7-chloro-3-methyl-2H-1,2,4-benzothiadiazine 1,1-dioxide | C8 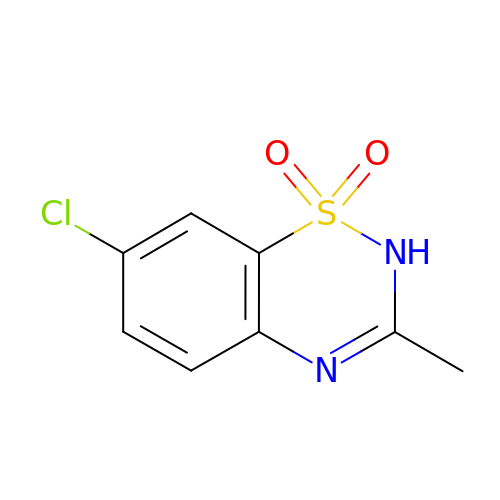H7 Cl N2 O2 S | GDLBFKVLRPITMI-UHFFFAOYSA-N>KREPALNPNEYKKFMLREKQIINHNTRLFRFNLHHPEDVVGLPIGQHMSVKATVDGKEIYRPYTPVSSDDEKGYFDLIIKVYEKGQMSQYIDHLNPGDFLQVRGPKGQFDYKPNMVKEMGMIAGGTGITPMLQVARAIIKN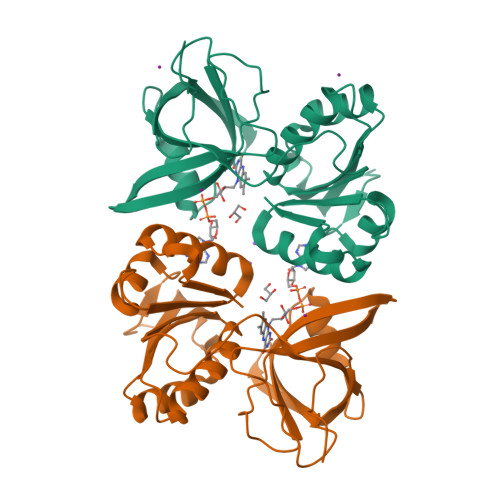PKEKTIINLIFANVNEDDILLRTELDDMAKKYSNFKVYYVLNNPPAGWTGGVGFVSADMIKQHFSPPSSDIKVMMCGPPMMNKAMQGHLETLGYTPEQWFIF[2x]>[2x]MKKGSANEDMPVERILEAELAVEPKTETYVEANMGLNPSSPNDPVTNICQAADKQLFTLVEWAKR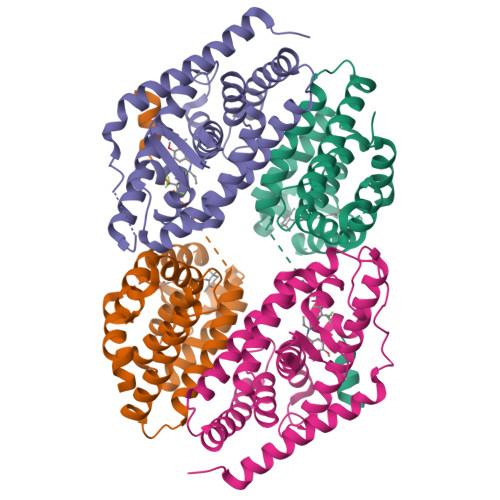IPHFSELPLDDQVILLRAGWNELLIASFSHRSIAVKDGILLATGLHVHRNSAHSAGVGAIFDRVLTELVSKMRDMQMDKTELGCLRAIVLFNPDSKGLSNPAEVEALREKVYASLEAYCKHKYPEQPGRFAKLLLRLPALRSIGLKCLEHLFFFKLIGDTPIDTFLMEMLEAPHQMT;>MRGSHHHHHHGMASLVPRGSVLPQLSPEQLGMIEKLVAAQQQCNRRSFSDRLRVTPWPIAPDPQSREARQQRFAHFTELAIVSVQEIVDFAKQLPGFLQLSREDQIALLKTSAIEVMLLETSRRYNPGSESITFLKDFSYNREDFAKAGLQVEFINPIFEFSRAMNELQLNDAEFALLIAISIFSADRPNVQDQLQVERLQHTYVEALHAYVSINHPHDPLMFPRMLMKLVSLRTLSSVHSEQVFALRLQDKKLPPLLSEIWDVHE[2x]>GSMAEAALEAVRRALQEFPAAARDLNVPRVVPYLDEPPSPLCFY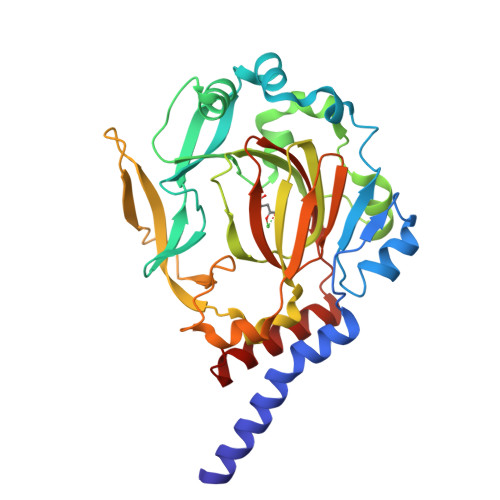RDWVCPNRPCIIRNALQHWPALQKWSLSYLRATVGSTEVSVAVTPDGYADAVRGDRFVMPAERRLPISHVLDVLEGRAQHPGVLYVQKQCSNLPTELPQLLSDIESHVPWASESLGKMPDAVNFWLGDASAVTSLHKDHYENLYCVVSGEKHFLLHPPSDRPFIPYNLYTPATYQLTEEGTFRVVDEEAMEKVPWIPLDPLAPDLTQYPSYSQAQALHCTVRAGEMLYLPALWFHHVQQSHGCIAVNFWYDMEYDLKYSYFQLMDTLTRATGLD[2x]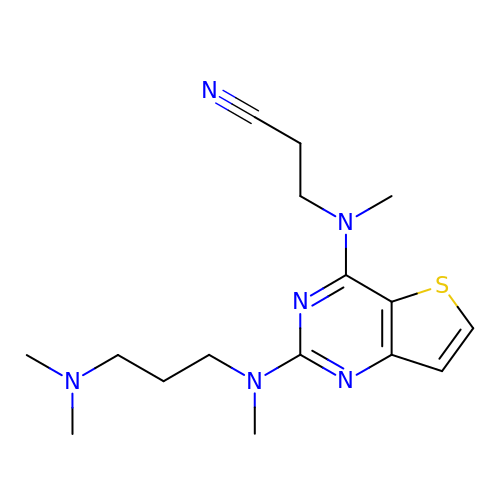3-[[2-[3-(dimethylamino)propyl-methyl-amino]thieno[3,2-d]pyrimidin-4-yl]-methyl-amino]propanenitrile | C16 H24 N6 S | JNFSCEZOWFOZJC-UHFFFAOYSA-N> MSQSNRELVVDFLSYKLSQKGYSWSQFSDVEENRTEAPEETEAERETPSAINGNPSWHLADSPAVNGATGHSSSLDAREVIP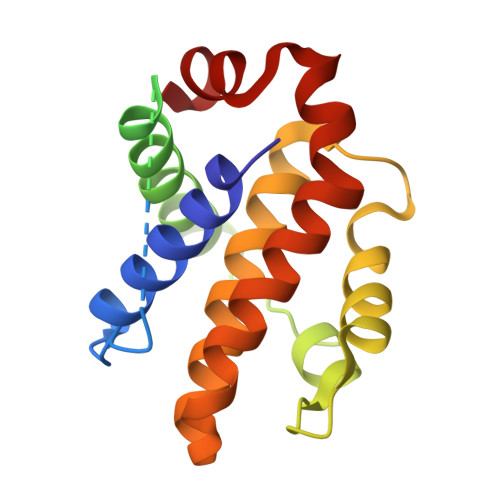MAAVKQALREAGDEFELRYRRAASDLTSQLHITPGTAYQSFEQVVNELFRDGVNWGRIVAFFSFGGALCVESVDKEMQVLVSRIASWMATYLNDHLEPWIQENGGWDTFVDLYG>[2x]MSSISLKEIIPPQPSTQRNFTTHLSYDPTTNAIAYPCGKSAFVRCLDDGDSKVPPVVQFTGHGSSVVTTVKFSPIKGSQYLCSGDESGKVIVWGWTFDKESNSVEVNVKSEFQVLAGPISDISWDFEGRRLCVVGEGRDNFGVFISWDSGNSLGEVSGHSQRINACHLKQSRPMRS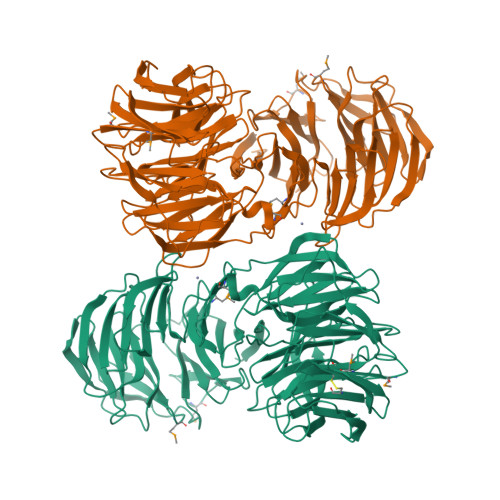MTVGDDGSVVFYQGPPFKFSASDRTHHKQGSFVRDVEFSPDSGEFVITVGSDRKISCFDGKSGEFLKYIEDDQEPVQGGIFALSWLDSQKFATVGADATIRVWDVTTSKCVQKWTLDKQQLGNQQVGVVATGNGRIISLSLDGTLNFYELGHDEVLKTISGHNKGITALTVNPLISGSYDGRIMEWSSSSMHQDHSNLIVSLDNSKAQEYSSISWDDTLKVNGITKHEFGSQPKVASANNDGFTAVLTNDDDLLILQSFTGDIIKSVRLNSPGSAVSLSQNYVAVGLEEGNTIQVFKLSDLEVSFDLKTPLRAKPSYISISPSETYIAAGDVMGKILLYDLQSREVKTSRWAFRTSKINAISWKPAEKGANEEEIEEDLVATGSLDTNIFIYSVKRPMKIIKALNAHKDGVNNLLWETPSTLVSSGADACIKRWNVVLE>[3x]ASTQGISEDLYNRLVEMATISQAAYADLCNIPSTIIKGEKIYNAQTDINGWILRDDTSKEIITVFRGTGSDTNLQLDTNYTLTPFDTLPQCNDCEVHGGYYIGWISVQDQVESLVKQQASQYPDYALTVTGHALGASMAALTAAQLSATYD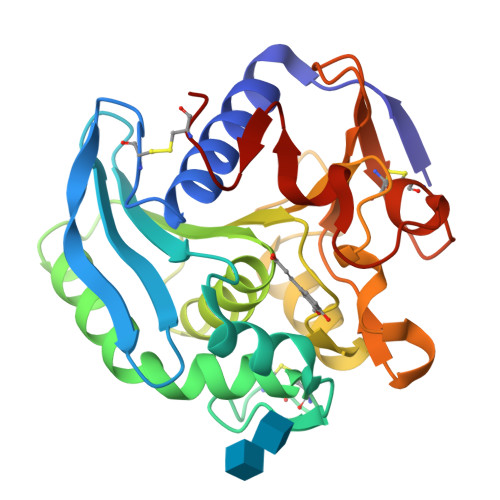NVRLYTFGEPRSGNQAFASYMNDAFQVSSPETTQYFRVTHSNDGIPNLPPADEGYAHGGVEYWSVDPYSAQNTFVCTGDEVQCCEAQGGQGVNDAHTTYFGMTSGACTW>[4x]MSNEIPKPVAPAPDILRCAYAELVVTDLAKSRNFYVDVLGLHVSYEDENQIYLRSFEEFIHHNLVLTKGPVAALKAMAFRVRTPEDVDKAEAYYQELGCRTERRKDGFVKGIGDALRVEDPLGFPYEFFFETTHVERLHMRYDLYSAGELVRLDHFNQVTPDVPRGRKYLEDLGFRVTEDIQDDEGTTYAAWMHRKGTVHDTALTGGNGPRLHHVAFSTHEKHNIIQICDKMGALRISDR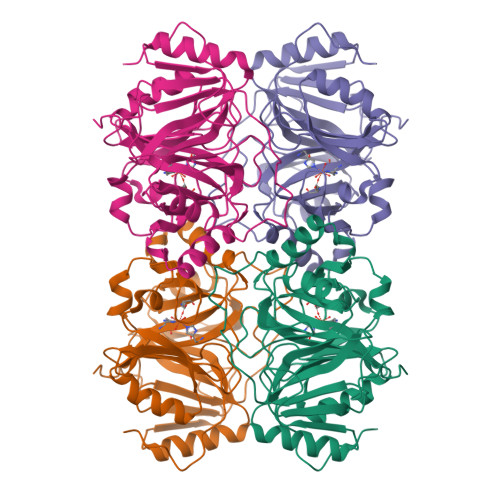IERGPGRHGVSNAFYLYILDPDNHRIEIYTQDYYTGDPDNPTITWNVHDNQRRDWWGNPVVPSWYTEASKVLDLDGNVQEII> MHHHHHHMNFNVSLMEKLKWKIKCIENKFLNYRLTTNETVVAETEYGKVKGVKRLTVYDDSYYSFEGIPYAQPPVGELRFKAPQRPTPWAGVRDCCNHKDKSVQVDFITGKVCGSEDCLYLSVYTNNLNPETKRPVLVYIHGGGFIIGENHRDMYGPDYFIKKDVVLINIQYRLGALGFLSLNSEDLNVPGNAGLKDQVMALRWIKNNCANFGGNPDNITVFGESAGAASTHYMMLTEQTRGLFHRGILMSGNAICPWANTQCQHRAFTLAKLAGYKGEDNDKDVLEFLMKAKPQDLIKLEEKVLTLEERTNKVMFPFGPTVEPYQTADCVLPKHPREMVKTAWGNSIPTMMGNTSYEGLFFTSILKQMPLLVKELETC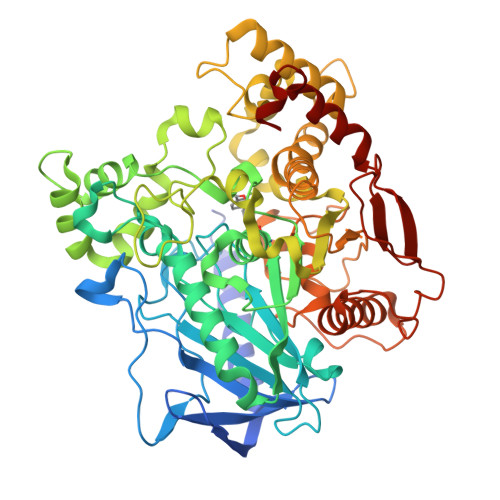VNFVPSELADAERTAPETLEMGAKIKKAHVTGETPTADNFMDLCSHFYFWFPMHRLLQLRFNHTSGTPVYLYRFDFDSEDLINPYRIMRSGRGVKGVSHTDELTYFFWNQLAKRMPKESREYKTIERMTGIWTQFATTGNPYSNEIEGMENVSWDPIEKSDEVYKCLNISDELKMIDVPEMGKIKQWESMFEKHRDLF>[4x]GSMAIDVDRTLAVLRRKLEALGYS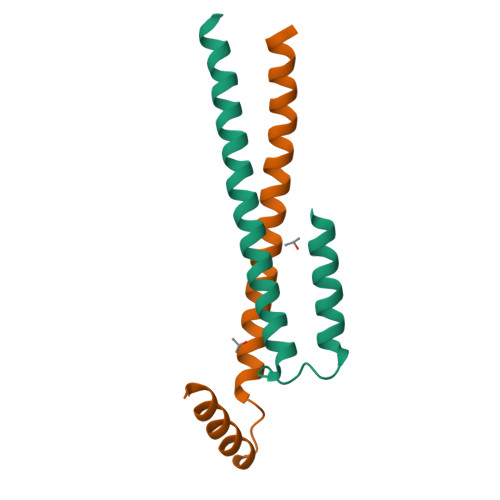DPLEPASLQLVQKLVEDLVHTTDSYTAVKQQCAKQAQEIAAFDTRLES>[2x]APEPIHPSHQQLNKRSLAYSEPHYPSPWMDPKAIGWEEAYEKAKAFVSQLTLLEKVNLTTGIGWGAEQCVGQTGAIPRLGLKSMCMQDAPLAIRGT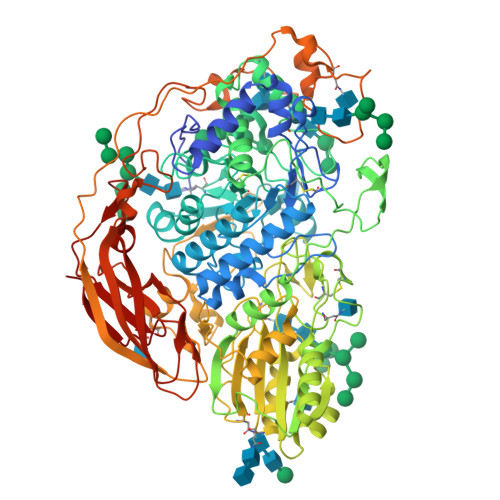DYNSVFPAGVTTAATFDRGLMYKRGYALGQEAKGKGVTVLLGPVAGPLGRAPEGGRNWEGFSTDPVLTGIAMAETIKGTQDAGVVACAKHFIGNEQEHFRQVGESQDYGYNISETLSSNIDDKTMHEMYLWPFVDAIRAGVGSFMCAYTQANNSYSCQNSKLLNNLLKQENGFQGFVMSDWQAHHSGVASAAAGLDMSMPGDTMFNSGRSYWGTNLTLAVLNGTVPQWRIDDMAMRIMAAFFKVGQTVEDQEPINFSFWTLDTYGPLHWAARKDYQQINWHVNVQGDHGSLIREIAARGTVLLKNTGSLPLKKPKFLAVIGEDAGPNPLGPNGCADNRCNNGTLGIGWGSGTGNFPYLVTPDQALQARAVQDGSRYESVLRNHAPTEIKALVSQQDATAIVFVNANSGEGFIEIDGNKGDRLNLTLWNEGDALVKNVSSWCNNTIVVLHTPGPVLLTEWYDNPNITAILWAGMPGQESGNSITDVLYGRVNPSGRTPFTWGATRESYGTDVLYEPNNGNEAPQLDYTEGVFIDYRHFDKANASVLYEFGFGLSYTTFEYSNLKIEKHQVGEYTPTTGQTEAAPTFGNFSESVEDYVFPAAEFPYVYQFIYPYLNSTDMSASSGDAQYGQTAEEFLPPKANDGSAQPLLRSSGLHHPGGNPALYDIMYTVTADITNTGKVAGDEVPQLYVSLGGPEDPKVVLRGFDRLRVEPGEKVQFKAVLTRRDVSSWDTVKQDWVITEYAKKVYVGPSSRKLDLEEVLP> ATGRPEWIWLALGTALMGLGTLYFLVKGMGVSDPDAKKFYAITTLVPAIAFTMYLSMLLGYGLTMVPFGGEQNPIYWARYADWLFTTPLLLLDLALLVDADQGTILALVGADGIMIGTGLVGALTKVYSYRFVWWAISTAAMLYILYVLFFGFTSKAESMRPEVASTFKVLRNVTVVLWSAYPVVWLIGSEGAGIVPLNIETLLFMVLDVSAKVGFGLILLRSRAIFGEAE

The primary function of bR is that of a light-driven proton pump, where trans to cis isomerization of a covalently bound retinal chromophore starts a series of conformational changes necessary for directional transport against a concentration gradient. Structurally, bR shares the seven trans-membrane α-helical topologies typical for other rhodopsins, as well as G protein-coupled receptors. The primary reaction from the bR dark state to the K-intermediate is the isomerization of retinal from the all-trans conformation to a twisted 13-cis conformation that stores a significant part of the initial photoenergy. Here, we investigate the effects of increasing laser power density on the light-driven proton pump bacteriorhodopsin with a focus on the K-intermediate that accumulates just after the excited retinal chromophore returns to the electronic ground state.

Reference difference density maps were recorded at 0.04 GW/cm2 with a nanosecond laser, for which direct multiphoton effects on the excited state are highly improbable, although the 13-cis retinal ground state may be photoexcited and return to an all-trans configuration. From these data, we observe the characteristic negative to positive density pairs corresponding to the move of retinal C20, as anticipated for the K-intermediate. Nevertheless, the positive differences around water 402 are also amplified, in agreement with the movement of water 402 in the nanosecond laser-derived K-intermediate at the lowest laser power density. We further rely on pairwise comparisons, for example, between the highest and lowest laser power settings used at SwissFEL, or by comparing femto- and nanosecond laser excitation under the same fluence at SACLA to reduce the impact of other experimental factors from measurements at different facilities. The overall structures are very similar in the temporal range from 6 ps to 16 ns where the K-intermediate of bR is dominant, as indicated by their low root mean square deviations (rmsd). On the purely structural level, our results show that even at the highest laser power densities, the overall conformation of the K-intermediate remained basically unchanged compared to structures obtained using nanosecond laser excitation and freeze-trapping experiments.1-(4-AMIDINOPHENYL)-3-(4-CHLOROPHENYL)UREA | C14 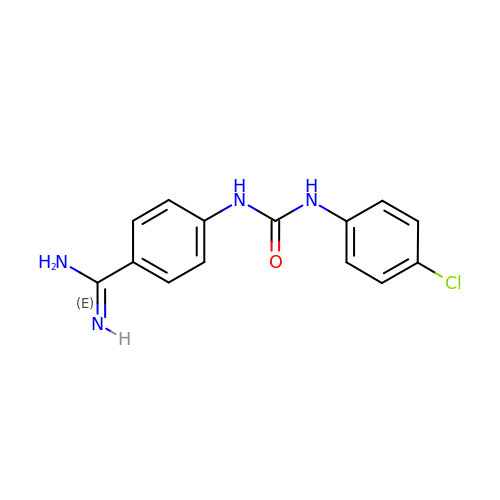H13 Cl N4 O | HQWKMDKTTCPCMQ-UHFFFAOYSA-N6-{[(3-fluorophenyl)methyl]sulfanyl}-2-(oxetan-3-yl)-5-phenyl-2,5-dihydro-4H-pyrazolo[3,4-d]pyrimidin-4-one 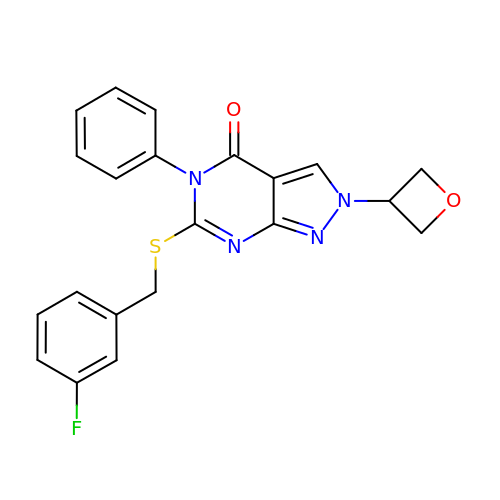| C21 H17 F N4 O2 S | IBYYWHNJSYBLSJ-UHFFFAOYSA-N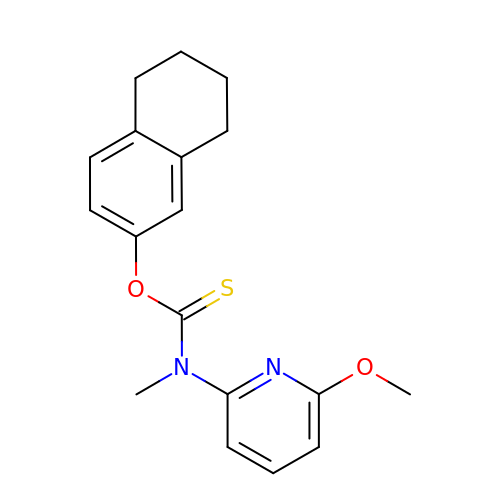~{O}-(5,6,7,8-tetrahydronaphthalen-2-yl) ~{N}-(6-methoxypyridin-2-yl)-~{N}-methyl-carbamothioate | C18 H20 N2 O2 S | VPHPQNGOVQYUMG-UHFFFAOYSA-N>GSYPPPVFDFGMPRNITTRTGHTAAINCRVDNLGDKSVSWIRKRDLHILTAGILTYTSDERFKVVRTADSKDWTLHVKYAQPRDSGIYECQVNTEPKISMAFRLNVIVTPPDAKAIIAGPTDLYVKVGSSVTLTCHVKQPATSAQDI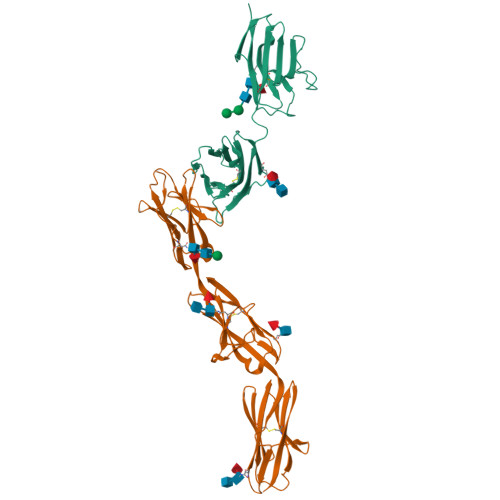GPIYWYRGPYILTPFVAHPNDAAIDLQRISMESTLAEKLQSRLRIANAQLLDTGNYTCMPTTAEAASVVVNVINDEHHHHHHHH[2x];>[2x]DLPKFGELLQNVTVPVSREAVLQCVVDNLQTYKIAWLRVDTQTILTIQNHVITKNHRMSITHAEKRAWILRIRDVKESDKGWYMCQINTDPMKSQVGYLDVVVPPDILDYPTSTDMVIREGSNVTLKCAATGSPTPTITWRREGGELIPLPNGAEAVAYNGSFLTIAKVNRLNMGAYLCIASNGIPPTVSKRVMLIVHFPPMIWIQNQLVGAALTQNITLECQSEAYPKSINYWMKNDTIIVPGERFVPETFESGYKITMRLTIYEVDIQDFGAYRCVAKNSLGDTDGAIKLYHIPHHHHHH>MTAAQGNSNETLFSSYKMGRFDLSHRVVLAPMTRCRALNGVPNAALAEYYAQRTTPGGFLISEGTMVSPGSAGFPHVPGIYSDEQVEAWKQVVEAVHAKGGFIFCQLWHVGRASHAVYQPNGGSPISSTNKPISENRWRVLLPDGSHVKYPKPRALEASEIPRVVEDYCLSALNAIRAGFDGIEIHGAHGYLIDQFLKDGINDRTDQYGGSIANRCRFLKQVVEGVVSAIGASKVGVRVSPAIDHLDATDSDPLSLGLAVVGMLNKLQGVNGSKLAYLHVTQPRYHAYGQTESGRQG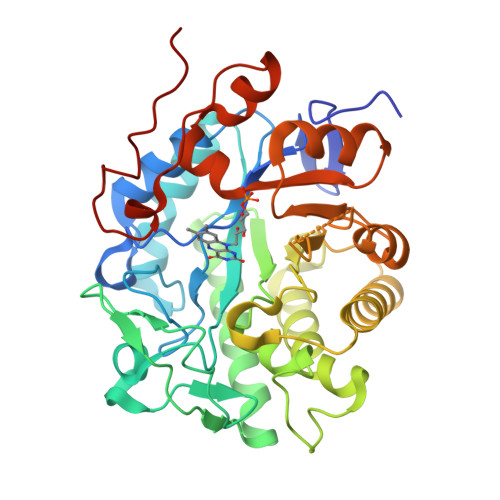SDEEEAKLMKSLRMAYNGTFMSSGGFNKELGMQAVQQGDADLVSYGRLFIANPDLVSRFKIDGELNKYNRKTFYTQDPVVGYTDYPFLAPFSRL[2x]>[2x]IVGGYTCEENSLPYQVSLNSGSHFCGGSLISEQWVVSAAHCYKTRIQVRLGEHNIKVLEGNEQFINAAKIIRHPKYNRDTLDNDIMLIKLSSPAVINARVSTISLPTAPPAAGTECLISGWGNTLSFGADYPDELKCLDAPVLTQAECKASYPGKITNSMFCVGFLEGGKDSCQRDAGGPVVCNGQLQGVVSWGHGCAWKNRPGVYTKVYNYVDWIKDTIAANS;>YVDYKDDDDKEVEVCSEQAEVGPCRARFSRWYFDVTEGKCAPFVYGGCGGNRNNFDTEEYCMAVCGSAIPRHHHHHHAAAN[2x]

To test our approach in a real-life context, we chose to map the binding selectivity landscape of a broad-spectrum trypsin inhibitor, namely, the human amyloid protein precursor inhibitor (APPI; a member of the human Kunitz-domain family of serine protease inhibitors), to each of the four human serine proteases—kallikrein-6 (KLK6), mesotrypsin, anionic trypsin, and cationic trypsin—all of which share high-sequence homology and structural similarity. APPI has attracted our interest as a scaffold for engineering selective serine protease inhibitors due to the marked sequence diversity among Kunitz family members, which possess canonical binding loops that are highly tolerant to substitution or incorporation of additional amino acids. Because the sequence of the canonical binding loop and neighboring residues largely determine the affinity and selectivity of the inhibitor to its targets, using APPI as a scaffold offers a unique opportunity to optimize target affinity and selectivity without compromising stability. We chose the serine protease family as an ideal group of targets to demonstrate our strategy mainly because inhibiting the human serine proteases is of clinical value: both KLK6 and mesotrypsin are involved in cancer progression, while anionic and cationic trypsins are involved in the etiology of pancreatitis.

We chose the KLK6-selective T11V/G17R and T11S/G17R double-mutant variants, and their corresponding single-mutant selectivity-switch variants T11V, T11S, and G17R. The amino acid substitution that most increased the total selectivity of APPI-3M toward KLK6 was T11V/G17R, followed by G17R and finally, T11S/G17R. The individual substitutions T11V and T11S did not improve the selectivity toward KLK6, rather they somewhat decreased it. These results suggest that residues 11 and 17 are correlated-selectivity residues, which act together to increase target selectivity. For example, we found that the mutations T11V and G17R, when combined, yield a highly potent and selective inhibitor for KLK6, while combining the mutations T11S and G17R yield only a moderately potent and partially selective inhibitor for KLK6. To gain insight into the structural basis of the observed selectivity changes, we attempted to crystallize the APPI-3M-T11V/G17R variant in complex with the increased-selectivity target KLK6 and the reduced-selectivity target mesotrypsin. A structural analysis of this complex revealed that a deleterious steric interaction between the APPI Arg-17 mutation and mesotrypsin Arg-193 pushes Arg-193 into a more buried conformation, as previously found in the structures of mesotrypsin bound to wild-type APPI or BPTI Kunitz-type inhibitors. The steric clash and the restriction of Arg-193 to a single buried conformation can explain the reduction in affinity toward mesotrypsin, which is consistent with our prior structure and mutagenesis studies.>MARFSIEGKSLKLDAITTEDEKSVFAVLLEDDSVKEIVLSGNTIGTEAARWLSENIASKKDLEIAEFSDIFTGRVKDEIPEALRLLLQALLKCPKLHTVRLSDNAFGPTAQEPLIDFLSKHTPLEHLYLHNNGLGPQAGAKIARALQELAVNKKAKNAPPLRSIICGRNRLENGSMKEWAKTFQSHRLLHTVKMVQNGIRPEGIEHLLLEGLAYCQELKVLDLQDNTFTHLGSSALAIALKSWPNLRELGLNDCLLSARGAAAVVDAFSKLENIGLQTLRLQYNEIELDAVRTLKTVIDEKMPDLLFLELNGNRFSEEDDVVDEIR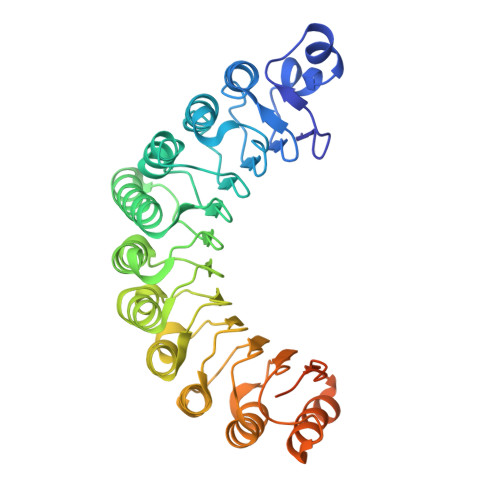EVFSTRGRGELDELDDMEELTDEEEEDEEEEAESQSPEPETSEEEKEDKELADELSKAHI[2x]> MEPAGRFTKVAAAVADSVVTIESVSDQEGMQGSGVIVDGRGYIVTNNHVISEAANNPSQFKTTVVFNDGKEVPANLVGRDPKTDLAVLKVDNVDNLTVARLGDSSKVRVGDEVLAVGAPLGLRSTVTQGIVSALHRPVPLAGEGSDTDTVIDAIQTDASINHGNSGGPLIDMDAQVIGINTAGKSLSDSASGLGFAIPVNEMKLVANS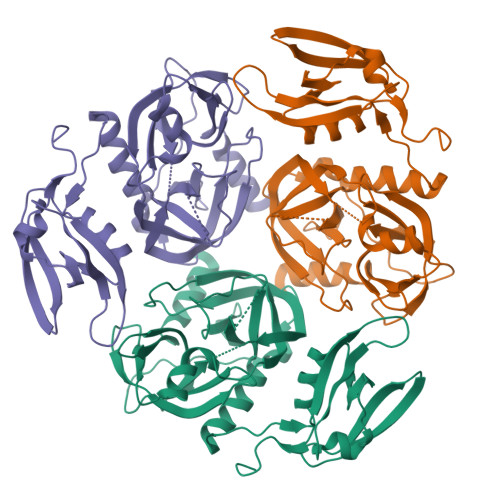LIKDGKIVHPTLGISTRSVSNAIASGAQVANVKAGSPAQKGGILENDVIVKVGNRAVADSDEFVVAVRQLAIGQDAPIEVVREGRHVTLTVKPDPDSTLEHHHHHH> CT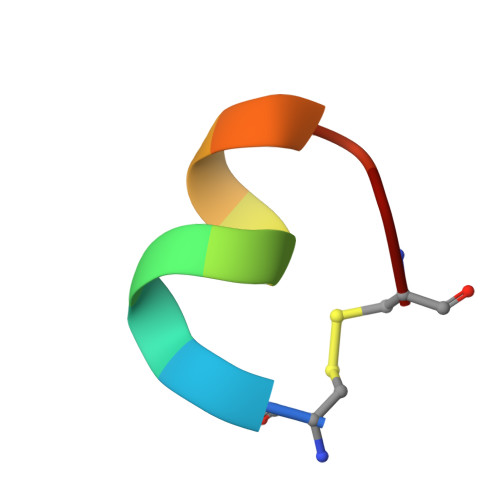ERMALHNLC> MKELFQKIWQNELQFLNFDAKFQDKSKLDTAECAIILSVNKDNYERYFLLKEFQELCKKIDLRV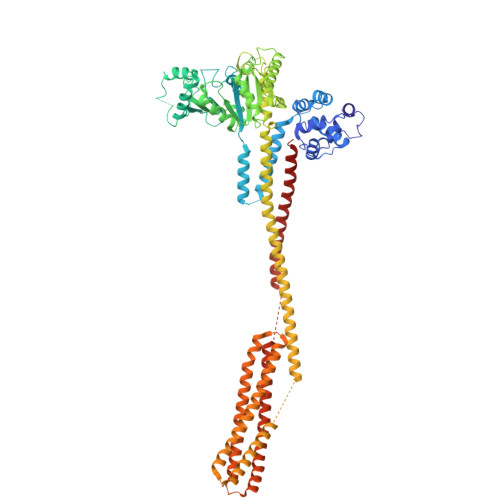DIFSMQNAQICILNLFKSGFISKQDLLKALKILEKISKNTEIFDFILQEKVQSIDQKALFQNDFKELNTINLELQKLSFDENLKSRLQKTLEKFQNLEFNIAITGVMNAGKSSLLNALLKEDFLGVSNIPETANLTVLSYGKSEEAKIYFWDKKEWQNILESSHFNADLKEFIDKLDKSVNIEDFIKDKPLIQNIALCELKNFSSAKNKISALIKKIEIKSHLEFLKNNISIVDTPGLDDVVVQREIVTNEYLRESDFLIHLMNASQSLTQKDADFLVHCLLNSRLSKFLIVLTKADLLSKKDLEEVIVYTKESLKSRLVDLDENLVEKIDFLCVSAKMASDFYKGLASKESLQKSGMQEFENYLFNELYAGEKSKIALRAYKKELHLELKNILSEYEMQNRLIKENKQGVSEENQKLLLELQKQNTLLKEAQDEISNSIAKLKNIDSGIDNLVLLLAKKLKERLIDEFKYLKNNAQKLNLSRILNIVDITTKDGINDILREIKFENIKKIEELKTNLSLKYDFLKDDFDNGFEGFKDGISKNIDSIFQSEKFALLRLKIEKLSNLKSDLYELETNLDTVIFDTFKEFKMSEILNSLNINGAFFEFLNDKLKHYEKNQKSKLESLEKVLQSLKNQDANILNSFEENLEKIEKLKQLEMGLLNADKLHH>MHHHHHHKYTVITGASSGIGYETAKLLAGKGKSLVLVARRTSELEKLRDEVKQISPDSDVILKSVDLADNQNVHDLYEGLKELDIETWINNAGFGDFDLVQDIELGKIEKMLRLNIEALTILSSLFVRDHHDIEGTTLVNISSAGGYRIVPNAVTYCATKFYVSAYTEGLAQELQKGGAKLRAKVLAPAATETEFADR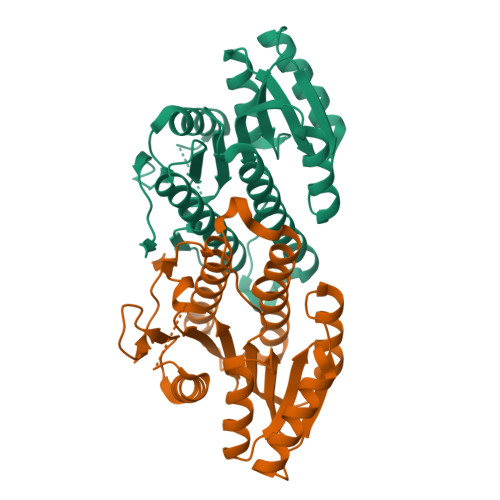SRGEAGFDYSKNVKKYHTAAEMAGFLHQLIESDAIVGIVDGETYEFELRGPLFNYAG[2x]> IVGGYTCGANTVPYQVSLNSGYHFCGGSLINSQWVVSAAHCYKSGIQVRLGEDNINVVEGNEQFISASKSIVHPSYNSETYNNDIMLIKLKSAASLNSRVASISLPTSCASAGTQCLISGWGNTKSSGTSYPDVLKCLKAPILSDSSCKSASSFIITSNMFCAGYLEGGKDACQGDSGGPV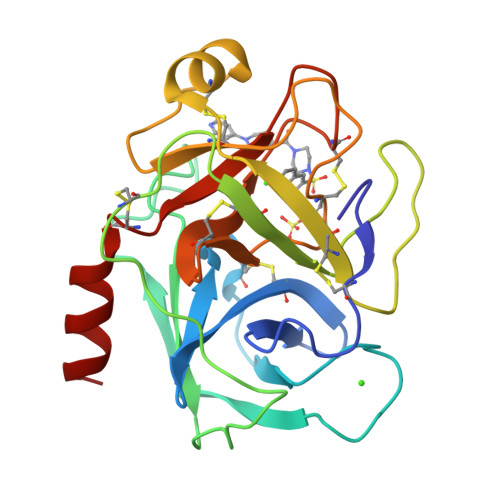VCSGKLQGIVSWGEGCAQKNKPGVYTKVCNYVSWIKQTIASN> MKLYRLTQKKFADTPFSPIGAKLFGKRWNSKGTEALYFSESESLCSLEVFVHVNNDPAITKLYDLYRIEMPEYLIATLDEEDLPVTWRAIPASESTQYIGDQFLNDPHPEFAALQVPSTISPRDKNYV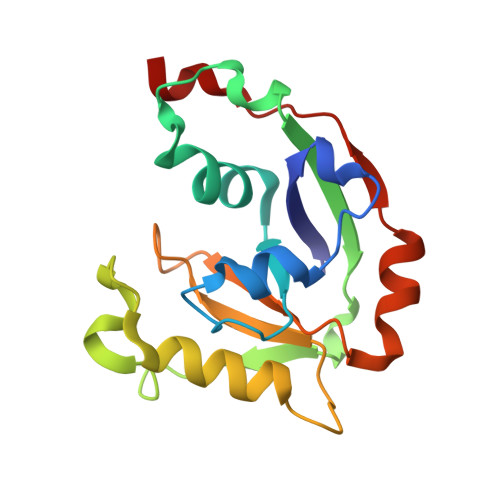VNPNHPKMKEIIKKAEKLDFAFDPRIFK3'-amino-2',3'-dideoxyguanosine 5'-(tetrahydrogen 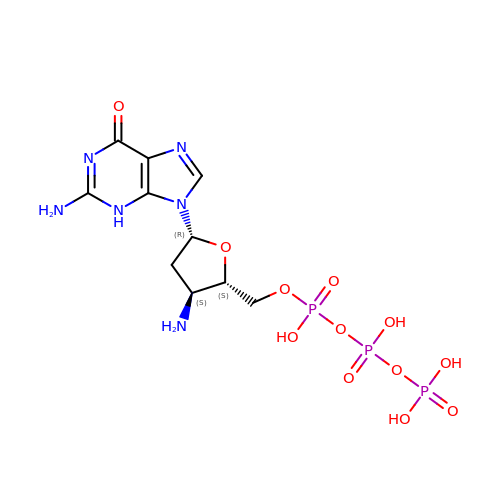triphosphate) | C10 H17 N6 O12 P3 | ILTYANYMUGEMNF-KVQBGUIXSA-N> PWGSMEFAKEIDVSYVKIEEVIGAGEFGEVCRGRLKAPGKKESCVAIKTLKGGYTERQRREFLSEASIMGQFEHPNIIRLEGVVTNSMPVMILTE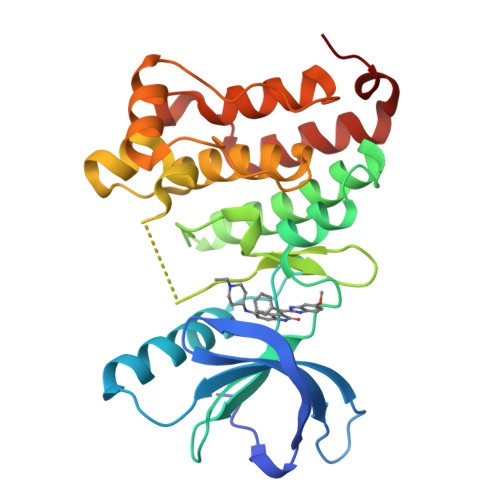FMENGALDSFLRLNDGQFTVIQLVGMLRGIASGMRYLAEMSYVHRDLAARNILVNSNLVCKVSDFGLSRFLEENSSDPTYTSSLGGKIPIRWTAPEAIAFRKFTSASDAWSYGIVMWEVMSFGERPYWDMSNQDVINAIEQDYRLPPPPDCPTSLHQLMLDCWQKDRNARPRFPQVVSALDKMIRNPASLKIVARE>[2x]MQEFEFAVPAPSRVSPDLARARARHLDWVHAMDLV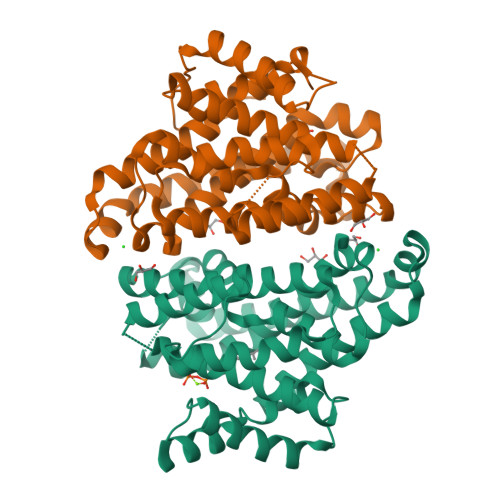RGEEARRRYEFSCVADIGAYGYPHATGADLDLCVDVLGWTFLFDDQFDAGDGRERDALAVCAELTDLLWKGTAATAASPPIVVAFSDCWERMRAGMSDAWRRRTVHEWVDYLAGWPTKLADRAHGAVLDPAAHLRARHRTICCRPLFALAERVGGYEVPRRAWHSSRLDGMRFTTSDAVIGMNELHSFEKDRAQGHANLVLSLVHHGGLTGPEAVTRVCDLVQGSIESFLRLRSGLPELGRALGVEGAVLDRYADALSAFCRGYHDWGRGASRYTTRDHPGDLGLENLVARSSG> MAELKLWEVFKDDFDIGAAVNVRTVDSAAELLRAQYNSITAENEMKPINTQPSEGVFTFEQADKIADFAAKHGKKLRGHTLVWHNQTPDWFFEAPGGGPAGKETLLRRMRDHIHAVAGRYKGRTYCWDVVNEAVADEGEQWLRASKWHDMVGPEFIVRAFEYAHEADPDALLFYNDYNECNPAKRDKIIRLVKWLKEQGAPIHGIGMQGHYNLASPSI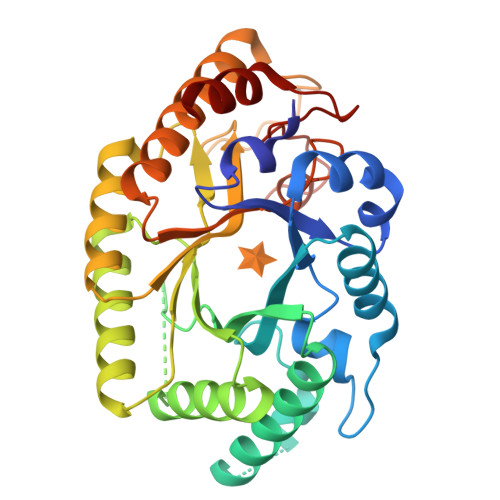AEVREAIEKYAELGLVIHVTELDMSVYAWDDRRTDLLEPTAEMVERQAELYEQLFSLYREYRDVIRSVTFWGAADDYTWLSYFPVRGRRNWPLLFDAQHRPKEAFRRVVRTAGAEA We have discovered, cloned, and characterized a fluorescent flavoprotein from a Geobacillus species that is homologous to other bacterial MurB enzymes. In the case of the Geobacillus-derived MurB homologue, FAD fluorescence is enhanced more than 10-fold, making this protein useful as a fluorescent fusion partner. We have named the novel MurB homologue LucY, for Lucigen Yellow. In a physiological setting, MurB catalyzes the reduction of uridine diphospho-N-acetylglucosamine enolpyruvate (UNAGEP) to UDP-N-acetylmuramic acid via a hydride transfer from NADPH to the substrate through FAD.

The high-resolution structure of LucY comprises 302 amino acid residues and displays a three-domain fold in complex with the FAD cofactor, similar to the previously published structures of related MurB enzymes. Domain 1 (N-terminal residues 1–83 and C-terminal 297–302) consists of two α-helices and six β-strands forming a four-stranded mixed β-sheet and a two-stranded parallel β-sheet. Domain 2 (residues 90 to 215) is formed by a five-stranded antiparallel β-sheet and three α-helices. Domain 3 (residues 235–288) contains a three-stranded antiparallel β-sheet and two α-helices. The binding-pocket of FAD is formed primarily by domains 1 and 2, with additional contributions from domain 3 and the loop connecting domains 2 and 3. One copy of the enzyme was observed per asymmetric unit, and the structure belongs to the trigonal space group R32. Interestingly, three crystallographic symmetry-related protein molecules formed an apparent fifteen-stranded β-barrel-like superstructure. Thus, we conclude that the fifteen-stranded β-barrel is a feature of the crystal packing instead of a true trimerization interface. All three magnesium ions in the structure are bound at the surface of the protein and appear to mediate crystal packing between symmetry-related molecules via interaction with the carboxylic groups of Asp 42 and Glu 286, amino groups of Lys 41 and backbone carbonyl groups of Lys 41, Glu 286, and Lys 287. Moreover, LucY, the brightest of the MurBs, does not contain a Trp or Tyr residue within 10 Å of its FAD binding pocket.

> MDKVIQELKDLQVGKVLENEPLANHTTIKIGGPADCLVIPKDIQAVRDTMEVVKNHGVQWRAIGRGSNLLVLDEGIRGVVIKLGAGLDHMEIDGEQVTVGGGYSVVRLSTGISKKGLSGLEFASGIPGSVGGAVYMNAGAHGSDISRILVKALILFEDGTMEWLTNEEMEFSYRTSILQNKRPGICLEAVLQLEQKERDAIVAQMQKNKDYRKETQPVSNPCAGSIFRNPLPDHAGRLVEQAGLKGHRIGGAKVSEMHGNFIVNAGGATAKDVLDLIAFIQKTIKEKYDIDMHTEVEIVGEKRHHHHHH>MNQSYGRLVSRAAIAATAMASLLLLIKIFAWWYTGSVSILAALVDSLVDIGASLTNLLVVRYSLQPADDNHS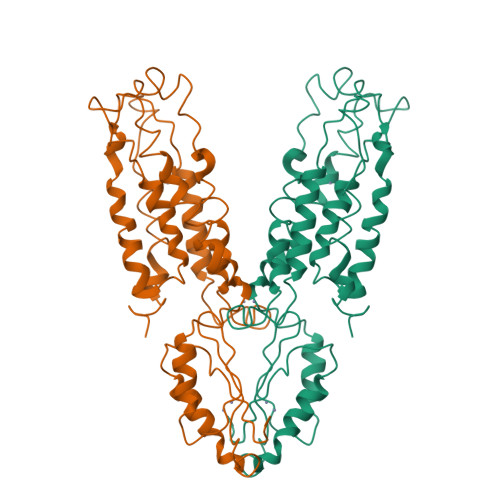FGHGKAESLAALAQSMFISGSALFLFLTGIQHLISPTPMTDPGVGVIVTIVALICTIILVSFQRWVVRRTQSQAVRADMLHYQSDVMMNGAILLALGLSWYGWHRADALFALGIGIYILYSALRMGYEAVQSLLDRALPDEERQEIIDIVTSWPGVSGAHDLRTRQSGPTRFIQIHLEMEDSLPLVQAHMVADQVEQAILRRFPGSDVIIHQDPCSVVPREGKRSMLS[2x]>[3x]GSHMASSVQPWSTIVQGPAESYVEFVNRLQISLADNLPDGVPKEP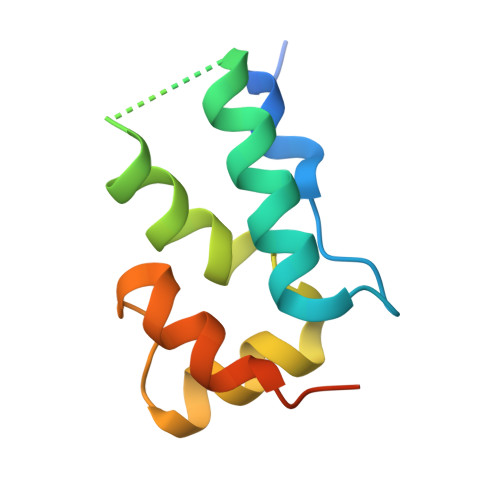IIDSLSYANANKECQQILQGRGLVAAPVGQKLQACAHWAPKVKQPAVL> GAMGSARRINDEIERQLRRDKRDARRELKLLLLGTGESGKSTFIKQMRIIHGSGYSDEDKRGFTKLVYQNIFTAMQAMIRAMDTLKIPYKYEHNKAHAQLVREVDVEKVSAFDV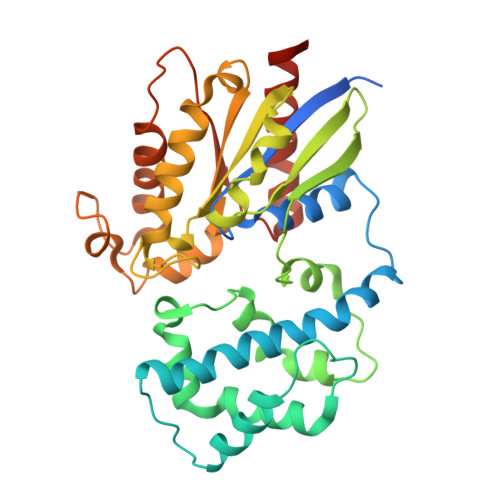PDYAAIKSLWNDPGIQECYDRRREYQLSDSTKYYLNDLDRVADPSYLPTQQDVLRVCVPTTGIIEYPFDLQSVIFRMVDVGGQRSERRKWIHCFENVTSIMFLVALSEYDQVLVESDNENRMEESKALFRTIITYPWFQNSSVILFLNKKDLLEEKIMYSHLVDYFPEYDGPQRDAQAAREFILKMFVDLNPDSDKIIYSHFTCATDTENIRFVFAAVKDTILQLNLKEYNLV>SNALEDSSTISFITWNIDGLDGCNLPERARGVCSCLALYSPDVVFLQEVIPPYCAYLKKRAASYTIITGNEEGYFTAILLKKGRVKFKSQEIIPFPNTKMMRNLLCVNVSLGGNEFCLMTSHLESTRGHSAERIRQLKTVLGKMQEAPDSTTVIFAGDTNLRDREVIKCGGLPDNVFDAWEFLGKPKHCQYTWDTKANNNLRIPAACKLRFDRIFFRAEEGHLIPQSLDLVGLEKLDCGRFPSDHWGLLCTLNVVL[2x]

Tyrosyl-DNA phosphodiesterase 2 (TDP2) {also known as TRAF and TNF receptor-associated gene (TTRAP) or ETS1-associated protein II (EAPII) } is a 5′-tyrosyl DNA phosphodiesterase that can remove the covalently-attached abortive complexes generated by DNA topoisomerase II (TOP2) when it is unable to complete its normal catalytic cycle. Fortunately, this type of DNA lesion is efficiently repaired, in part though the action of TDP2, which hydrolyses the phosphotyrosyl bond in a magnesium cofactor-dependent reaction, leaving ligatable 5′-phosphate moieties. Consequently, TDP2 has attracted interest as a target for small molecule inhibitors that might have utility in overcoming innate or acquired resistance to TOP2 poisons. Using a ‘humanized’ mouse TDP2 expression construct, we have now determined X-ray crystal structures of the catalytic domain of TDP2 in complex with deazaflavin inhibitors, revealing the unusual molecular interactions underpinning their mode of action.

We therefore created the expression construct m2hTDP2CAT (m2h=mouse-‘to’-human) by mutating the following mouse residues to their human equivalent: E242G, Q278R, Y321C and H323L. The m2hTDP2CAT protein retained full phosphodiesterase activity, and consistent with our prediction that the resistance of the mouse protein to deazaflavins was due to the variant M7-motif, this activity in m2hTDP2CAT was inhibited by 163. We were able to validate our approach, by determining the X-ray crystal structure of m2hTDPCAT bound to 163, at a resolution of 1.8 Å. Superposition of the low-resolution hTDP2CAT and high-resolution m2hTDP2CAT structures in complex with 163, confirms that the binding site is conserved across both proteins. However, the higher resolution data obtained with the m2hTDP2CAT surrogate, allows a far more detailed characterization of the interaction of the inhibitor with the TDP2 catalytic domain. The guanidinium head group of Arg276 (all numbering is for the mouse protein, the equivalent in human is calculated by subtraction of 10) is involved in an extensive hydrogen-bond network, including both carbonyl and nitrogen groups of the 163 pyrimido-dione ring, as well as the backbone carbonyl and side chain (via a water molecule) of Asp277. As in the fully human protein, amino acids of the M7-motif coalesce to form the ‘hydrophobic-shelf’, which permits extensive van der Waals interactions with the tricyclic deazaflavin core; these residues include Trp307, Ile317, Ala319, Cys321 (text in italics represent a ‘humanized’ amino acid residue), Leu323 and Phe325. The tetrazole R1 substituent of 163, is directed towards solvent, but packs against the carbon-atoms of the Arg241 side chain, providing additional van der Waals interactions.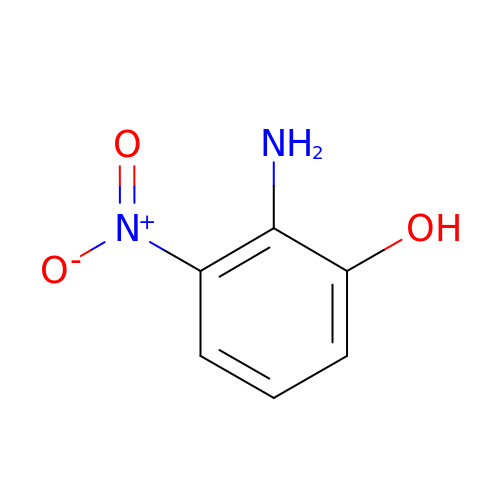2-azanyl-3-nitro-phenol | C6 H6 N2 O3 | KUCWUAFNGCMZDB-UHFFFAOYSA-N> MAHHHHHHMIREILKMGDPRLLEVAKPVAQFDTPELHEIVADMFETMHHANGAGLAAPQIGIGLQIIIFGFGSNNRYPDAPPVPETVLINPKLEYMPPDMEEGWEGCLSVPGMRGVVSRYAKVRYSGYDQFGAKIDRV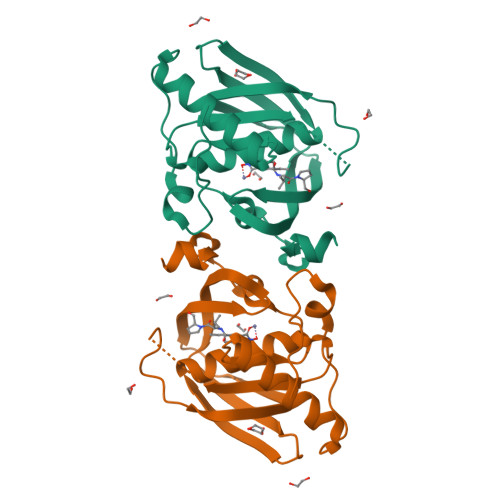AEGFHARVVQHEYDHLIGKLYPMRITDFTRFGFTEVLFPGLDPTDDD Human Shieldin consists of four subunits, REV7 (also known as MAD2L2 or MAD2B, 211 residues), SHLD1 (205 residues), SHLD2 (835 residues), and SHLD3 (250 residues). As the first identified member of the Shieldin complex, REV7 is composed entirely of a HORMA domain, acting as an interaction module in a broad array of cellular pathways. The Shieldin complex acts as the key downstream effector of 53BP1; it not only binds and shields single-stranded DNA ends but also mediates CST- and Polα-dependent fill-ins of DNA breaks. TRIP13 forms a hexamer to drive the REV7-mediated disassembly of Shieldin in an adenosine triphosphate (ATP)-dependent manner, thereby releasing the DSB DNA ends for resection to promote HDR.

To test whether REV7 can adopt a dimeric alignment in its complexes with SHLD peptides, we next designed a fusion protein containing an SHLD2 fragment (residues 1 to 19) fused through a Gly–Ser linker to an SHLD3 fragment (residues 1 to 58) and a C-terminal fragment of REV3 (residues 1887 to 1894) (labeled SHLD2.3). The structure of this SHLD2.3–Rev74 complex was solved at 3.8-Å resolution (X-ray statistics in SI Appendix) and is shown in two orientations. The crystallographic asymmetric unit contains one SHLD2.3–REV74 complex composed of a pair of REV7 conformational heterodimers connected by a pair of head-to-head aligned SHLD2.3–SHLD2.3 β-sheets. In each REV7 conformational heterodimer, one REV7 adopts an open (O-REV7) while the other exhibits a closed (C-REV7) conformation. The SHLD2.3 fusion protein serves as a strap with its N and C termini binding O-REV7 and C-REV7, respectively, therby strengthening the conformational heterodimerization of REV7. The 936 Å2 dimeric interface between O-REV7 and C-REV7 is further mediated by multiple intermolecular hydrophobic and hydrogen bonding interactions. Notably, Arg-124 of O-REV7 forms hydrogen bonds with Ala-135 of C-REV7, while Arg-124 of C-REV7 forms hydrogen bonds with Glu-35 of O-REV7, highlighting the importance of Arg-124, consistent with previous reports. The C-REV7 forms the typical safety-belt including an intact β8′/β8″ hairpin, identical to that observed in the SHLD3s–REV7 complex, while O-REV7 lacks both the safety belt and the β8′ strand. The β1 strand of SHLD2 is positioned between the β6 strand of O-REV7 (antiparallel alignment) and the β1 strand of SHLD3 (parallel alignment) as shown in Fig. 2 G and H, with this sandwiched β-sheet topology stabilized by hydrophobic and hydrogen bonding interactions. We anticipate that REV7 tetramerization reflects the short SHLD2(residues 1 to 19) segment used in the fused SHLD2.3 construct, which on replacement by the longer SHLD2L(residues 1 to 52) in the SHLD2L.3 construct would disrupt the tetramerization interface due to the presence of additional β2 and β3 segments of SHLD2.

>[4x]STTLTRQDLNFGQVVADVLCEFLEVAVHLILYVREVYPVGIFQKRKKYNVPVQMSCHPELNQYIQDTLHCVKPLLEKNDVEKVVVVILDKEHRPVEKFVFEITQPPLLSISSDSLLSHVEQLLRAFILKISVCDAVLDHNPPGCTFTVLVHTREAATRNMEKIQVIKDFPWILADEQDVHMHDPRLIPLKTMTSDILKMQLYVEERAHKGS;>[2x]MSQVHIFWGAPIAPLKGSGSGSGSGSGSGSGSTTEVILHYRPCESDPTQLPKIAEKAIQDFPTRPLSRFIPWFPYDGSKLPLRPKRSPPASREEIMATL>MNHKVHHHHHHIEGRHMPDDLNAVVTELDKEGVKYKISPDGRTIYVPENVARELRLKLAAKGVPRKGIVGYELFDKSGIVLSRFQQLVNFKRAIEGELAKTIMSLDCVEFARVHIVLPEKSLFIREEEEAKASVFLKLKPGCELTPEQVKAIRNLVSGSVENLKPSQVVVVDD[2x]

The MS-ring is a transmembrane ring assembly of a single protein, FliF, and has a two-tier ring structure; the S-ring is an upper ring located in the periplasm, and the M-ring is a lower ring embedded in the inner membrane. FliF is a 60-kDa protein with a large periplasmic region between two transmembrane helices. The MS-ring provides a base for the assembly of the flagellar structure. Previous sequence analysis revealed that the periplasmic region of FliF has three ring-building motifs (RBMs), namely, RBM1, RBM2, and RBM3, which are conserved in SctJ/SctD, SctJ/SctD/SpoIIIAH, and SpoIIIAG, respectively.

Therefore, we prepared FliF fragments from a thermophilic bacterium, A. aeolicus, and determined the crystal structure of a fragment consisting of residues 58 to 213 (Aa-FliF58–213) at 2.3-Å resolution. The crystal belongs to the space group of H3 and contains two essentially identical molecules in an asymmetric unit (the root mean square deviation for Cα atoms is 0.694). The structure of Aa-FliF58–213 consists of two distinct domains corresponding to RBM1 (D1; Pro58 to Ser122) and RBM2 (D2; Arg123 to Asp213). The D1 domain (FliFD1) is a compact globular domain composed of two α-helices (α1 and α2) and five β-strands (β1 to β5). β1, β2, and β3 form a core β sheet flanked by the two α-helices and another β-sheet made up of β4 and β5. The D2 domain (FliFD2) is more elongated and consists of two α-helices (α3 and α4) and four β-strands (β6 to β8 and βi). An intramolecular disulfide bridge is formed between C147 and C182 at a pole of FliFD2 but is not essential for the FliF function, as discussed later. Aa-FliF58–213 forms a dimer related by a pseudo-2-fold symmetry in the crystal, and β4 and β5 form an intersubunit β sheet with βi of the dimer mate. However, the dimer is a crystal-packing artifact because FliF forms a ring structure, and the 2-fold symmetrical dimer cannot be fitted in the cryoEM density, as shown later. We found that FliFD1 shows structural similarity to both PrgKD1 and PrgHD2, although the N-terminal α-helix of FliFD1 (α1) is longer than the corresponding helix of PrgHD2. FliFD2 resembles both PrgKD2 and PrgHD3, which adopt a common RBM fold.N-({(2E)-2-[(4-bromophenyl)methylidene]hydrazino}carbonothioyl)-beta-D-glucopyranosylamine | C14 H18 Br N3 O5 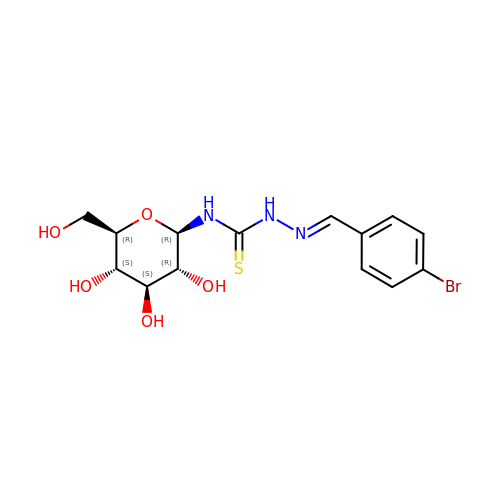S | BNLZUNIPJMEPID-QCOQDYPWSA-N>[4x]SMLLQGKVALITGAASERGIGRATAEIFAQQGAKVIIVDLDLAQSQNAAKALGEGHMGLAANVANEEQVKAAVEQALQHYGKIDILIN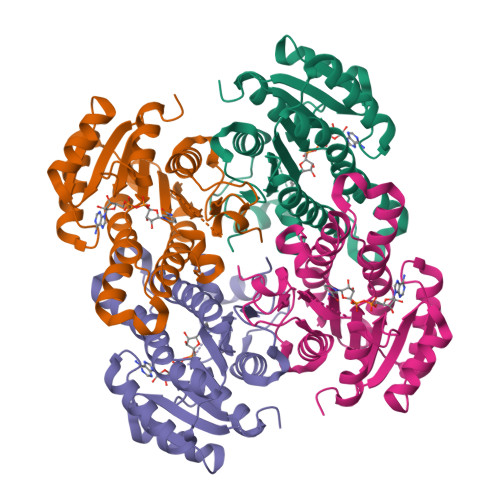NAGITQPIKTLDIQRSDYDRVLDVSLRGTLIMSQAVIPSMKANGGGSIVCLSSVSAQRGGGIFGGPHYSAAKAGVLGLAKAMAREFGGDQIRVNSLTPGLIQTDITGGLMNDDRRHDILAGIPLGRLGKAQDVANAALFLASDLSAYLTGVTLDVNGGMLIH>[18x]MAESVHLYLKANGSDIKGDSTQTSLGRADSIECVAYSQKVFTAREAGSGLATGRRQYEGIEITKRIDKSSPLLMKALCENQVIDATFKFFRPNPTGDGTTEQFYTVSIKKARINAIQQTVPNSFVPASTNLPPMETLQLVFHTINWTITQGGVTHEDTWDTQR;>[18x]MSKESSVAPTERVNIVYKPATGNAQEQVELPLKVLMLGDFTGQEDARPLEQRAPINVDKANFNEVMAQQNLKVTLTAADKLSADPNATMNVSLQFKNLNDFSPESVVNQVPELKKLLELRSALNALKGPLGNLPAFRKKLQALLADEDGRKALIKELGLTEETK;>[18x]MANETQTQKSTGVANDASLSLLDEILSEAKLKPKDEGYDVAKRGVQAFITEMLAPNRSEERVDKALVDAMIAEIDKRLSSQVNEILHAKEFQKLE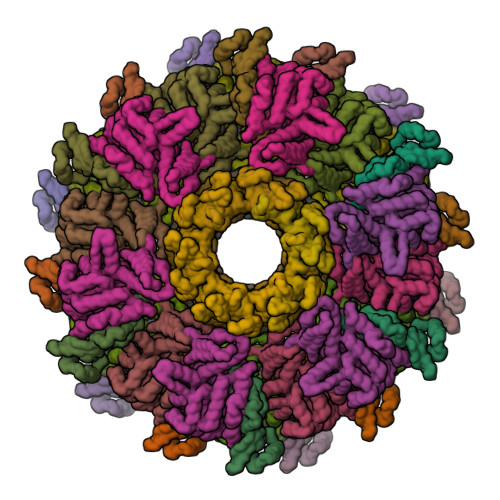SSWRSLKFMVDRTDFRENTRVEMLNASKEDLQKDFEDAPEVTKSGLYKLVYSNEYGVFGGKPYGIISANYDFNVGPQDMELLRKCASVAAMAHAPFIGNAAPEVFGEESFLKLPDLKDLKSLFEGPQYARWHSFRESEDARYVGLALPRFLLRLPYGEKTVPVKAFNFTEDVVGHHERYLWGHASVALTSRVADSFAKFRWSPNIIGPQSGGAVENLPLHQYEAMGEIQTKIPTEVMLTERREFELSEEGFIGLVFRKDSDNAAFFSANSTQKPRFFGNTPEGKAAETNYRLGTQLPYMFIMTRLAHYIKVLQREQIGSWKEKSDLERELNHWLSQYISDMDDPAPAVRSRRPLRAARVVVEDVEGQPGWYRCSLQVRPHFKYMGASFTLSLVGKLDKE> GPKKTDPELAEKINEMLDVILEYKNEDGELIADVFQTLPTRKELPD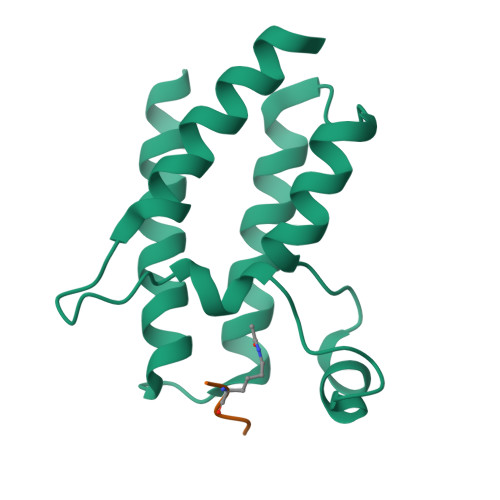YYQVISKPMDFDRINKKIETGRYTVMEELNDDMNLLVNNAQTYNEEGSEIYVSSETIGKLWKEQYDKFMNPPKPVEE;> ARKSTGGKAPRKQL> ASNSLQYVNVQVKDIEADLQHGVDESYTLDVEEDSDTITINAETVWGALHAFTTLQQLVISDGHGGLIIEEPVNIKDSPLYPYRGIMLDTGRNFVSLPKIFEQLEGMSLSKLNVLHWHIDDAQSWPIWVDVYPEMVKDAYSPHEIYSRNDVRNIVNYARARGIRVIPEIDMPSHSSSGWKQVDPEMVTCTDSWWSNDDWPLHTAVEPNPGQLDIIYNK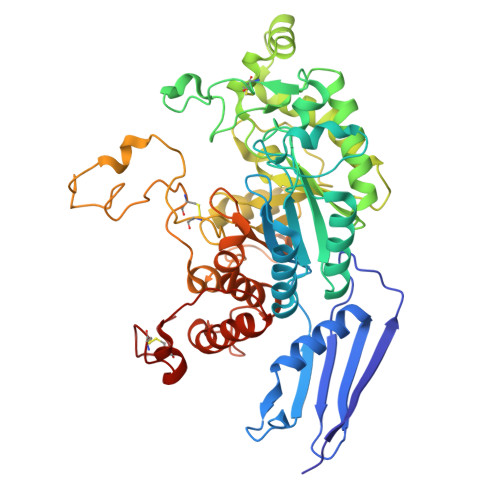TYEVVGNVYKELSDIFPDHWFHVGGDEIQPNCFNFSTHVTKWFAEDPSRTYHDLAQYWVDHAVPIFQNYSQERRLVMWEDIALSADNAHDVPKNIVMQSWNNGLEYISNLTARGYDVIVSSSDFLYLDCGHGGFVTNDPRYNVMANPDANTPNFNYGGNGGSWCAPYKTWQRIYDYDFTLNLTETQAKHIIGATAPLWGEQVDDINVSSMFWPRAAALAELVWSGNRDANGNKRTTEMTQRILNFREYLVANGVQAQALVPKYCLQHPHACDLYRNQAAIQ> S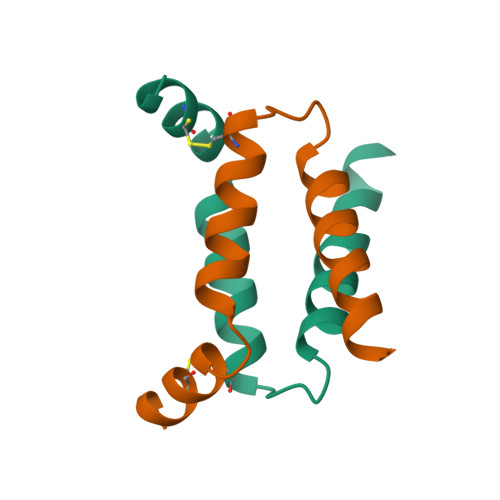LRECELYVQKHNIQALLKDSIVQLCTARPERPMAFLREYFEKLEKEEAK> SELYHAQIHLYKHVYNFVSSMALKSAMELGIADAIHNHG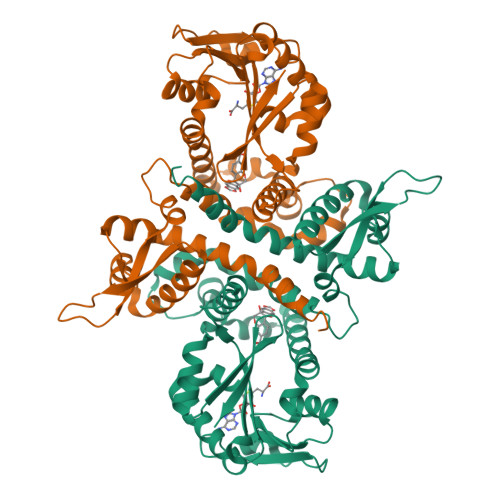KPMTLSELASSLKLHPSKVNILHRFLRLLTHNGFFAKTIVKGKEGDEEEEIAYSLTPPSKLLISGKPTCLSSIVKGALHPSSLDMWSSSKKWFNEDKEQTLFECATGESFWDFLNKDSESSTLSMFQDAMASDSRMFKLVLQENKRVFEGLESLVDVGGGTGGVTKLIHEIFPHLKCTVFDQPQVVGNLTGNENLNFVGGDMFKSIPSADAVLLKWVLHDWNDEQSLKILKNSKEAISHKGKDGKVIIIDISIDETSDDRGLTELQLDYDLVMLTMFLGKERTKQEWEKLIYDAGFSSYKITPISGFKSLIEVYP>SNAQDTCFLAKENQTVLKREGNDCDQRYSPASTFKIALSLMGFDSGILKDELHPEWPYKKEYELYLNVWKYPQNPHTWIRDSCVWYSQALTRQLGMKRFKGYVDAFHYGNQDVSGDKGQNNGLTHAWLSSSLSISPTEQIQFLQKIIYKKLPVSQKAYTMTKNIMYIQELPGGWKLYGKTGTGRQLTKDKSQKLPLQHGWFVGWIEK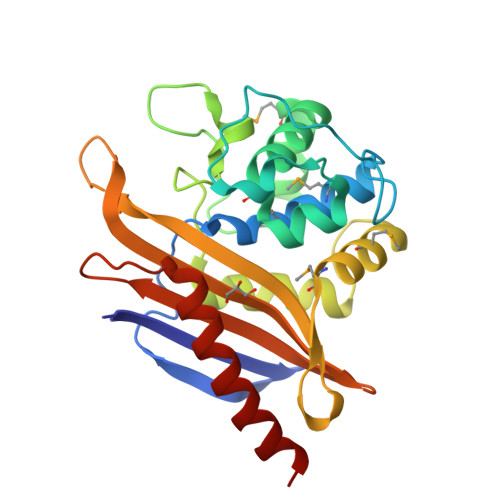DERVITFAKHIADSKENTTFASFRAKNDTLIQLFNLINELEK[12x]> TIQPGTGYNNGYF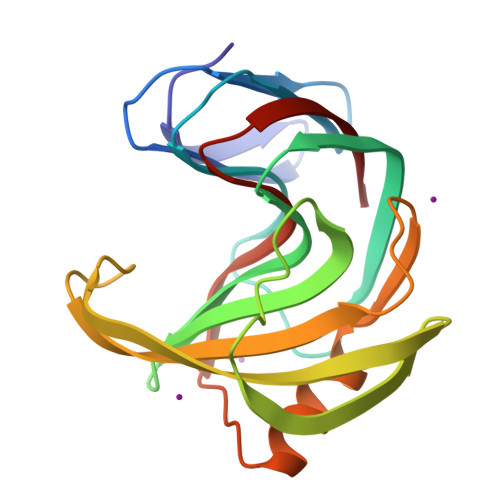YSYWNDGHGGVTYTNGPGGQFSVNWSNSGNFVGGKGWQPGTKNKVINFSGSYNPNGNSYLSVYGWSRNPLIEYFIVENFGTYNPSTGATKLGEVTSDGSVYDIYRTQRVNQPSIIGTATFYQYWSVRRNHRSSGSVNTANHFNAWAQQGLTLGTMDYQIVAVEGYFSSGSASITVS> MSNAKERKHAKKMRNQPTNVTLSSGFVADRGVKHHSGGEKPFQAQKQEPHPGTSRQRQTRVNPHSLPDPEVNEQSSSKGMFRKKGGWKAGPEGTSQEIPKYITASTFAQARAAEISAMLKAVTQKSSNSLVFQTLPRHMRRRAMSHNVKRLPRRLQEIAQKEAEKAVHQKKEHSKNKCHKARRCHMNRTLEFNRRQKKNIWLETHIWHAKRFHMVKKWGYCLGERPTVKSHRACYRAMTNRCLLQDLSYYCCLELKGKEEEILKALSGMCNIDTGLTFAAVHCLSGKRQGSLVLYRVNKYPREMLGPVTFIWKSQRTPGDPSESRQLWIWLHPTLKQDILEEIKAACQCVEPIKSAVCIADPLPTPSQEKSQTELPDEKIGKKRKRKDDGENAKPIKKIIGDGTRDPCLPYSWISPTTGIIISDLTMEMNRFRLIGPLSHSILTEAIKAASVHTVGEDTEETPHRWWIETCKKPDSVSLHCRQEAIFELLGGITSPAEIPAGTILGLTVGDPRINLPQKKSKALPNPEKCQDNEKVRQLLLEGVPVECTHSFIWNQDICKSVTENKISDQDLNRMRSELLVPGSQLILGPHESKIPILLIQQPGKVTGEDRLGWGSGWDVLLPKGWGMAFWIPFIYRGVRVGGLKESAVHSQYKRSPNVPGDFPDCPAGMLFAEEQAKNLLEKYKRRPPAKRPNYVKLGTLAPFCCPWEQLTQDWESRVQAYEEPSVASSPNGKESDLRRSEVPCAPMPKKTHQPSDEVGTSIEHPREAEEVMDAGCQESAGPERITDQEASENHVAATGSHLCVLRSRKLLK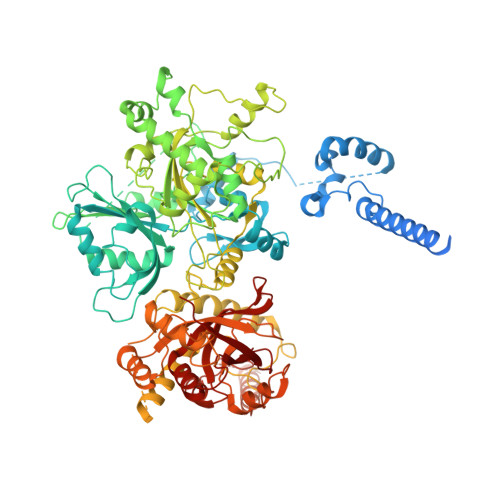QLSAWCGPSSEDSRGGRRAPGRGQQGLTREACLSILGHFPRALVWVSLSLLSKGSPEPHTMICVPAKEDFLQLHEDWHYCGPQESKHSDPFRSKILKQKEKKKREKRQKPGRASSDGPAGEEPVAGQEALTLGLWSGPLPRVTLHCSRTLLGFVTQGDFSMAVGCGEALGFVSLTGLLDMLSSQPAAQRGLVLLRPPASLQYRFARIAIEV Several rice NLR immune receptors, including RGA5, possess an integrated heavy metal–associated (HMA) domain that recognizes corresponding Magnaporthe oryzae Avrs and ToxB-like (MAX) effectors in the rice blast fungus. Interestingly, RGA5 and Pik1 encode NLR immune receptors with a HMA domain, which acts as an ID directly binding corresponding MAX Avr effectors and mediates their helper NLR receptor–triggered immunity. The rice NLR immune receptor RGA5 recognizes corresponding MAX effectors AVR1-CO39 and AVR-Pia by its HMA domain (25–27).

The RGA5-HMA2 domain is contrived based on the high structural similarity of AvrPib with two MAX effectors, AVR-Pia and AVR1-CO39, recognized by cognate RGA5-HMA, the binding interface between AVR1-CO39 and RGA5-HMA, and the distinct surface charge of AvrPib and RAG5-HMA. Therefore, we reasoned that the mutation causing two amino acid substitutions (S1027V and G1009D) in the interface of the RGA5-HMA domain might interact with AvrPib while decreasing the binding ability to AVR1-CO39. V1027 of HMA2 could form the hydrophobic interaction with V27 of AvrPib, while it could affect the interaction with Y40 of AVR1-CO39. The G-to-D mutation at 1,009 of HMA2 could repel D35 of AVR1-CO39 while forming the salt bridge with R23 of AvrPib. Since there is a positively charged patch on the surface of AvrPib, the C-terminal K-rich region of the HMA domain would have blocked the interaction between RGA5-HMA and AvrPib. To circumvent the issue, we generated the RGA5-HMAK/E variant (K to E mutations including K at the 1,071, 1,073, 1,080, 1,081, 1,085, and 1,086 sites). However, no interaction was detected between RGA5-HMAK/E and AvrPib. Finally, we contrived another RGA variant, RGA5-HMAS1027V, G1009D, K/E (henceforth RGA5-HMA2), by combining all the above mutations, which were confirmed to resemble the native RGA5-HMA structure. Again, we performed a Y2H assay, which showed that RGA5-HMA2 could interact with AvrPib but not with AVR-Pia, implying that the mutations in RGA5-HMA2, which do not affect the conformation of the domain, acquire the binding affinity to the originally unrecognized MAX effector AvrPib. The data obtained from the MST assays also confirmed the interaction between RGA5-HMA2 and AvrPib, which displayed a dissociation constant (Kd) of 148 μM, compared to 31 μM for the RGA5-HMA/AVR-Pia interaction.

>RTKIVVKVHMPCDKSRAKAMALAASVNGVDVVEITGEDKDRLVVVGRGIDPVRLVALLREKCGLAELLMVELV[14x]> XVDVA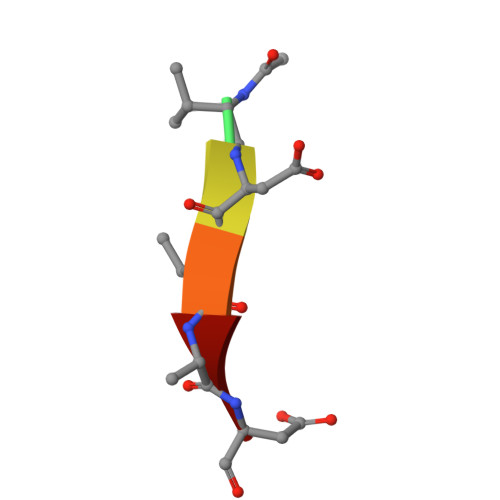D> MAKTPMRVAVTGAAGQICYSLLFRIANGDMLGKDQPVILQLLEIPNEKAQKALQGVMMEIDDCAFPLLAGMTAHADPMTAFKDADVALLVGARPRGPGMERKDLLEANAQIFTVQGKAIDAVASRNIKVLVVGNPA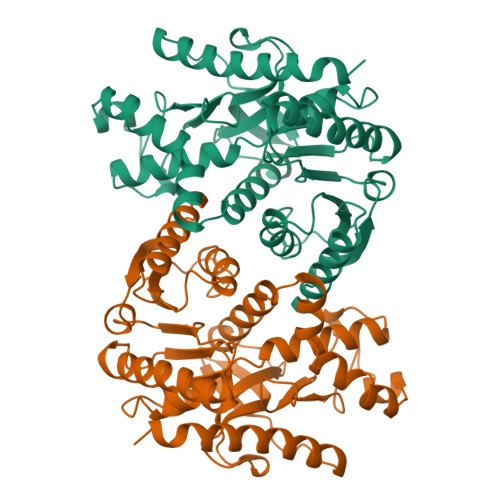NTNAYIAMKSAPSLPAKNFTAMLRLDHNRALSQIAAKTGKPVSSIEKLFVWGNHSPTMYADYRYAQIDGASVKDMINDDAWNRDTFLPTVGKRGAAIIDARGVSSAASAANAAIDHIHDWVLGTAGKWTTMGIPSDGSYGIPEGVIFGFPVTTENGEYKIVQGLSIDAFSQERINVTLNELLEEQNGVQHLLG>GPKPKNTKENLSKSSWRQEWLANLKLISVSLVDEFPSELSDSDRQIINEKMQ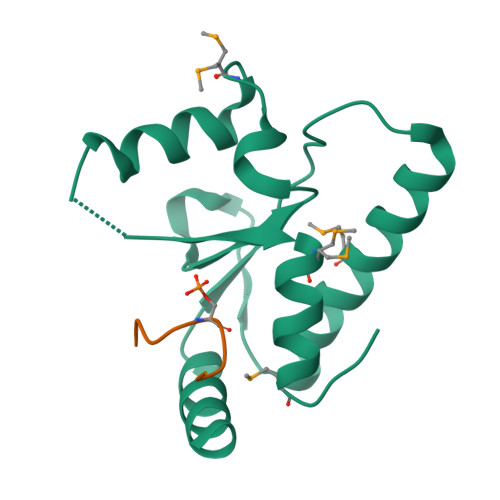LLKDIFANNLKSAISNNFRESDIIILKGEIEDYPMSSEIKIYYNELQNKPDAKKARFWSFMKTQRFVSNMGFDIQ[8x];>[8x]IPSTDLPSDPPSDKEE> QYAPQTQSGRTSIVHLFEWRWVDIALECERYLGPKGFGGVQVSPPNENIVVTNPSRPWWERYQPVSYKLCTRSGNENEFRDMVTRCNNVGVRIYVDAVINHMCGSGAAAGTGTTCGSYCNPGNREFPAVPYSAWDFNDGKCKTASGGIESYNDPYQVRDCQLVGLLDLALEKDYVRSMIADYLNKLIDIGVAGFRIDASKHMWPGDIKAVLDKLHNLNTNWFPAGSRPFIFQEVIDLGGEAIKSSEYFGNGRVTEFKYGAKLGTVVRKWSGEKMSYLKNWGEGWGFMPSDRALVFVDNHDNQRGHGAGGASILTFWDARLYKIAVGFMLAHPYGFTRVMSSYRWARNFVNGEDVNDWIGPPNNNGVIKEVTINADTTCGNDWVCEHRWREIRNMVWFRNVVDGEPFANWWDNGSNQVAFGRGNRG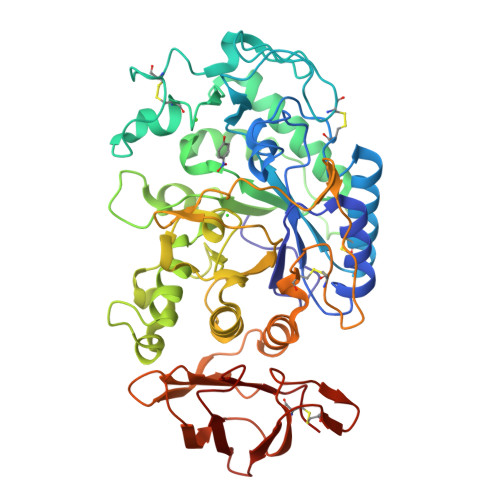FIVFNNDDWQLSSTLQTGLPGGTYCDVISGDKVGNSCTGIKVYVSSDGTAQFSISNSAEDPFIAIHAESKL>[2x]MMTDLSTPDLPRMSAAIAEPTSHDPDSGGHFGGPSGWGGRYVPEALMAVIEEVTAAYQKERVSQDFLDDLDRLQANYAGRPSPLYEATRLSQHAGSARIFLKREDLNHTGSHKINNVLGQALLARRMGKTRVIA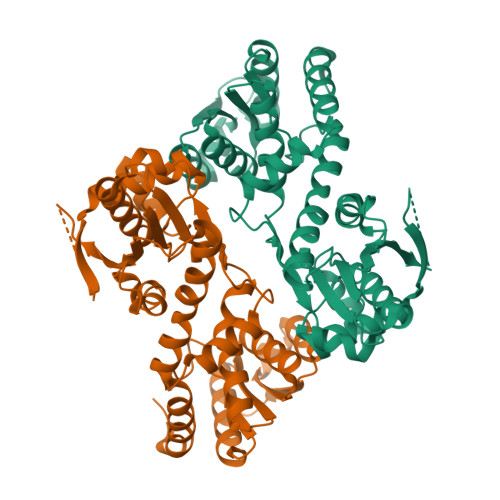ETGAGQHGVATATACALLGLDCVIYMGGIDTARQALNVARMRLLGAEVVAVQTGSKTLKDAINEAFRDWVANADNTYYCFGTAAGPHPFPTMVRDFQRIIGMEARVQIQGQAGRLPDAVVACVGGGSNAIGIFHAFLDDPGVRLVGFEAAGDGVETGRHAATFTAGSPGAFHGSFSYLLQDEDGQTIESHSISAGLDYPGVGPEHAWLKEAGRVDYRPITDSEAMDAFGLLCRMEGIIPAIESAHAVAGALKLGVELGRGAVIVVNLSGRGDKDVETAAKWFGLLGND Mycobacteria synthesize intracellular polymethylated polysaccharides (PMPS) of 6-O-methylglucose (MGLP) and of 3-O-methylmannose (MMP), both proposed to sequester and protect newly formed fatty-acyl CoA chains in the cytoplasm, thus modulating fatty acid (FA) metabolism and indirectly the lipidic cell envelope. MMP is composed of a linear chain of 11 to 14 units of α-(1→4)-linked 3-O-methyl-D-mannose (3-O-MeMan), blocked in the reducing end by a methyl aglycon, and with an unmethylated mannose at the nonreducing end. Using a combination of MMP purification and chemoenzymatic syntheses of intermediates, we identified the biosynthetic mechanism of MMP, relying on two enzymes that we characterized biochemically and structurally: a previously undescribed α–endomannosidase that hydrolyses MMP into defined-sized mannoligosaccharides that prime the elongation of new daughter MMP chains by a rare α-(1→4)-mannosyltransferase. In this elegant mechanism, MmpH serves as the recycling enzyme that hydrolyses mature MMP into defined-size smaller oligomannosides that are, in turn, substrates for ManT and MeT1 activities for further processing into new daughter MMP chains.

The three-dimensional structure of MmpH was determined at 1.35 Å resolution from monoclinic (space group P21) crystals. Although there are two MmpH molecules in the asymmetric unit of the crystals, the enzyme behaves as a monomer in solution, as suggested both by size exclusion chromatography and DLS analysis, and underscored by assessment of the protein contacts in the crystal using PISA26. MmpH is globular and mostly α-helical, with a diameter of approximately 45 Å. Thirteen α-helices (αA-αM) are arranged into two concentric layers to form an (α/α)6-barrel. At the center of the (α/α)6-barrel there is a deep cavity, opening to the exterior at one of the ends of the barrel. The catalytic base (Glu628 in G1d and Glu393 in CpGH125) seems to be conserved in MmpH (Glu262), as is the network of solvent molecules coordinated to these residues and that participate in the inverting reaction mechanism. In agreement, replacing Glu262 of MmpH with an alanine residue completely abolished its activity. The drastic reduction of activity observed for both Asp47Ala and Asp50Ala MmpH variants is compatible with one of these residues being the catalytic acid. Interestingly, in MmpH the volume corresponding to those residues is part of its large depression and could accommodate an additional sugar moiety, in line with its endo-mannosidase activity and in contrast with the exo-mannosidase properties of GH125 family members.

>MVLRDDLDAVPGVPGVLTPEQCRQTAQAIADAQEPSGALPWFEGGHTDPWDHVENAMALTVAGLLEPARAAFDWCRTTQRPDGSWPIQIRNGVVEDANSDSNFCAYVATGVWHHVLITGDRRFAETMWPVVAKAIDFVIDMQLPGGEIAWARSPSGLYEEALLTGCASIYHSIRCALALADYMGEPQPEWEVAVGRLGHAIAEHPEAFVTKDRWSMEWYYPVLGGALRGEAARARINRRWNDFVVPGLGIRCVDDRPWVTGAETCELVLALDAIGDLTRAHEQFAAMHHLREEDGSYWTGLVYDDGKRWPIERTTWTGAAMILAADALSRTTPGNGIFRGVDLPRGLEGEYDCACATSERKLAAALEHHHHHH[2x]> MSNEDYGYDYDYLFKIVLIGDSGVGKSNLLSRFTTDEFNIESKSTIGVEFATRTIEVENKKIKAQIW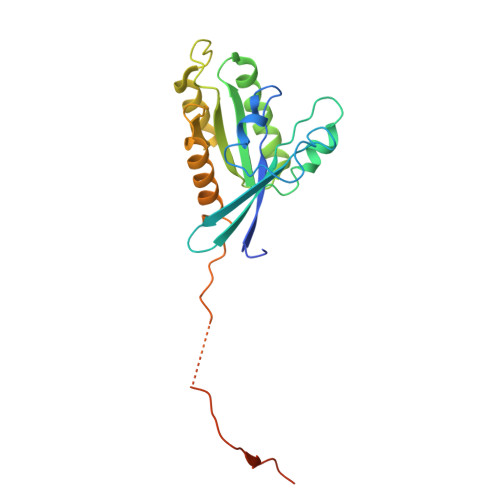DTAGQERYRAITSAYYRGAVGALIVYDISKSSSYENCNHWLTELRENADDNVAVGLIGNKSDLAHLRAVPTDEAKNFAMENQMLFTETSALNSDNVDKAFRELIVAIFQMVSKHQVDLSGSGTNNMGSNGAPKGPTISLTPAPKEDKKKKSSNHHHHHHH>[3x]KTGNGTVSVGKKGKERQIVHVGAGEISDTSTDAVNGSQLHALATVVAQNKADIKDLDDEVGLLGEEINS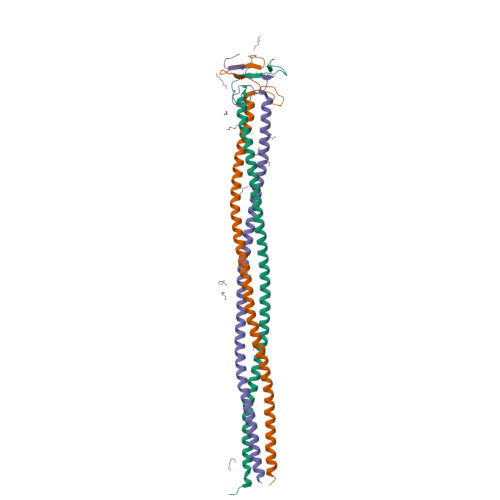LEGEIFNNQDAIAKNQADIKTLESNVEEGLLDLSGRLLDQKADIDNNINNIYELAQQQDQHSSDIKTLKNNVEEGLLDLSGRLIDLVPR> MQKSDEVTEKFKRYCNQLEKYGQTENVHSPVMAMLRRKGRKQLIEIMKRDGDCTSSINKLWIVGYYHP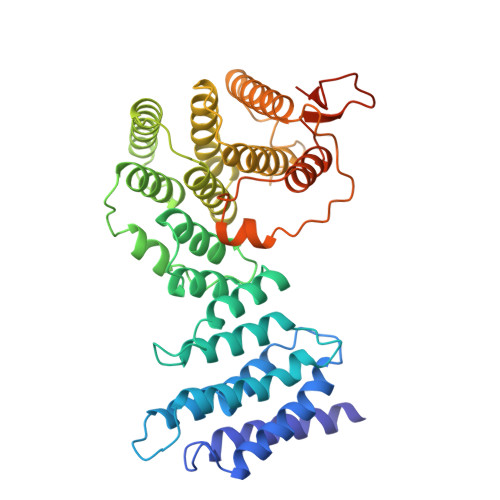FQFFIRDKEKNMAIAVLLTMFCGELQEMLSLPDDKYPALWNMYIGDFHRYMPDEEIQKCLAVGYYSRAIDLDPNQGRAFHVLAGLRADLNVAQKLRLMILGQLADAPYKKGTELLEYLKFPQKESTDKLMVDFVIWALNEKSKRMDYQMTGIKIVNEFKAEIEQKLEFDWSLIMSTCRLASKLAMKKFGFQQFYNCFDTISTLYITIYSRTISSKCLLAEAISWISDSAEILGHLDEQKNEPHFQKLSVFAKTKWNELNDLVMNHINSVFTSMSLTINPSISMTSFLLNGPISEPNVEFLSQLINYLVSVEFPPMEIIHDREESGPLLRRINQSEQKRLDIQIKTQNDEVNR> MHHHHHHSTATNPLDLDVCAREPIHIPGLIQPYGVLLVIDPADGRIVQASTTAADLLGVPMAALLGMPYTQVLTLPEAQPFAVDDQPQHLMHAEVRFPQRATPPASAWVAAWHLYPQQWLVEMEPRDARLLDVTLREAMPLLRSVERDPGIAEAAVRVAKGLRSLI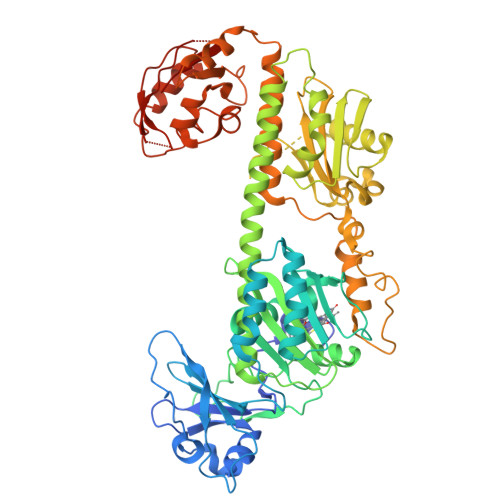GFDRVMIYRFDEEWNGDIIAEARKPELEAYLGLHYPASDIPAQARALYLRNRVRQIADVGYQPSPIQPTVHPQLGTPVDLSDVSLRSVSPVHLEYLANMGVTATLVASIVVNDALWGLISCHHYSPHFTNHAMRDVTDAVARTLAGRIGALQAVARARLESVLLTVREKLITDFNDAEHMTVELLDDMAPDLMDVVDADGVAIFHGNDISRHGTTPDVAALRRIRDHIESEHHEALREDAVGALHVDAIGEVFPELADLAPLAAGFIFVPLMPQSRSALLWTRREQIQQIKWAENPQLAKLEDIPNSRLSPRKSFDLWQQTVRGRARRWSPLHLESARSLRVLIELMERKRFQQDFTLLEASLSRLRDGVAIIERGTANAAHRLLFVNTAFADVCGSDVAELIGRELQTLYASDAPRANVELLQDALRNGRAAYVTLPLQVSDGAPVYRQFHLEPLPSPSGVTAHWLLQLRDPE>[2x]CGSSSHETSYGY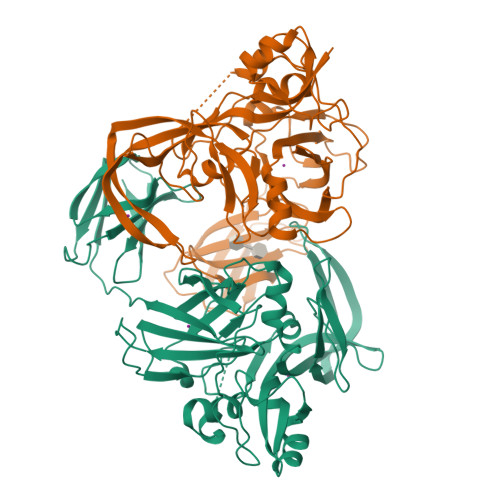ATLSYADYWAGELGQSRDVLLAGNAEADRAGDLDAGMFDAVSRATHGHGAFRQQFQYAVEVLGEKVLSKQETEDSRGRKKWEYETDPSVTKMVRASASFQDLGEDGEIKFEAVEGAVALADRASSFMVDSEEYKITNVKVHGMKFVPVAVPHELKGIAKEKFHFVEDSRVTENTNGLKTMLTEDSFSARKVSSMESPHDLVVDTVGTGYHSRFGSDAEASVMLKRADGSELSHREFIDYVMNFNTVRYDYYGDDASYTNLMASYGTKHSADSWWKTGRVPRISCGINYGFDRFKGSGPGYYRLTLIANGYRDVVADVRFLPKYEGNIDIGLKGKVLTIGGADAETLMDAAVDVFADGQPKLVSDQAVSLGQNVLSADFTPGTEYTVEVRFKEFGSVRAKVVAQ> GSMVPPPENVRMNSVNFKNILQWESPAFAKGQLTFTAQYLSYRIFQDKCMQTTLTECDFSSLSKYGDHTLRVRAEFADEHSDWVQITFCPVDDTIIGPPGMQVEVLADSLHMRFLAPKIENEYETWTMKNVYNSWTYNVQYWKQGTDEKFQITPQYDFEVLRNLEPWTTYCVQVRGFLPDRNKAGEWSEPVCEQTTHDETVPSAAAHHHHHHHH;> TSRRPRLAPPQNVTLLSQNFSVYLTWLPGLGNPQDVTYFVAYQSSPTRRRWREVEECAGTKELLCSMMCLKKQDLYNKFKGRVRTVSPSSKSPWVESEYLDYLFEVEPAPPVLVLTQTEEILSANATYQLPPCMPPLDLKYEVAFWKEGAGNKTLFPVTPHGQPVQITLQPAAS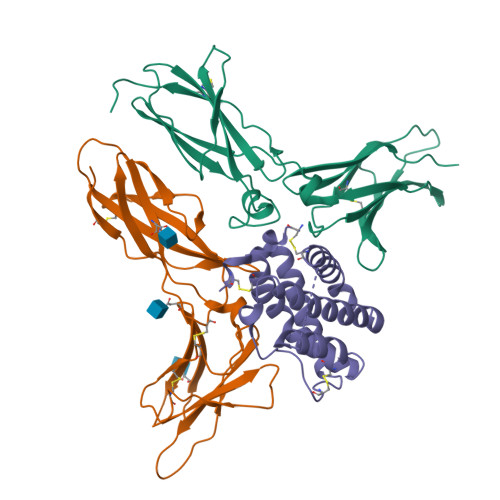EHHCLSARTIYTFSVPKYSKFSKPTCFLLEVPEANAAALEVLFQ;> GSARGCHIAQFKSLSPRELQAFKRAKDALEESLLLKDCKCRSRLFPRTWDLRQLQVRERPVALEAELALTLKVLDATADTDPALGDVLDQPLHTLHHILSQLRACIQPQPTAGPRTRGRLHRWLHRLQEAPKKESPGCLEASVTFNLFRLLARDLNCVASGDLCEAAAHHHHHHHH>[2x]MFTGSIVAIVTPMDEKGNVCRASLKKLIDYHVASGTSAIVSVGTTGEFATL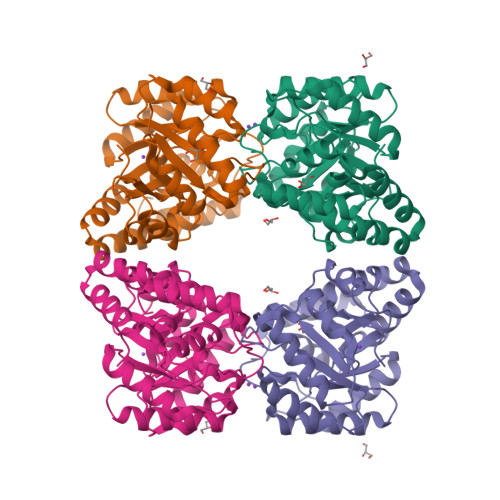NHDEHADVVMMTLDLADGRIPVIAGTGANATAEAISLTQRFNDSGIVGCLTVTPYYNRPSQEGLYQHFKAIAEHTDLPQILYNVPSRTGCDLLPETVGRLAKVKNIIGIKEATGNLTRVNQIKELVSDDFVLLSGDDASALDFMQLGGHGVISVTANVAARDMAQMCKLAAEGHFAEARVINQRLMPLHNKLFVEPNPIPVKWACKELGLVATDTLRLPMTPITDSGRETVRAALKHAGLL> SNAIDPVMVAAFEGWNDAGDAASTAVAHLDREWKGEVFAALDAEDYYDFQVNRPTVWLDGGVRKITWPTTRLSVVRVGGEKPRDLVLVRGIEPSMRWRSFCNELLAFAHELGVELVVVLGALLGDTPHTRPVPVSGVTSDPDLARTMDLEETKYEGPTGIVGILQEACTHAGVPAVSLWAAVPHYVSQPPNPKATLALLNRL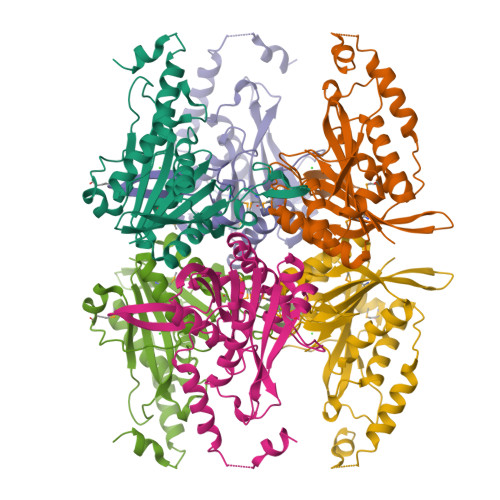EDLIDVRIPLGELPEDARAWQVGVDQLAAEDSEVAEYVQSLEEARDTA>[4x]LMLHKRNICPIKGCGKNFFSHKYLVQHQRVHSDDRP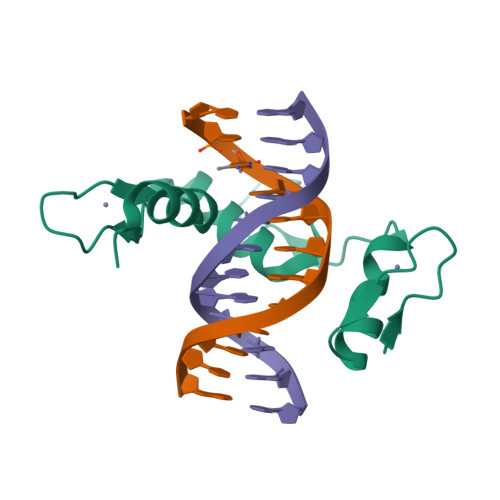LKCPWKGCKMTFKWAWSRTEHIRVHTGARPYVCAEPDCGQTFRFVSDFSRHKRKTGHSVKKTNKR>[4x]TEKKYIVALDQGTTSSRAVVMDHDANIISVSQREFEQIYPKPGWVEHDPMEIWATQSSTLVEVLTKADISSDQIAAIGITNQRETTIVWEKETGKPIYNAIVWQCRRTAEICEHLKRDGLEDYIRSNTGLVIDPYFSGTKVKWILDHV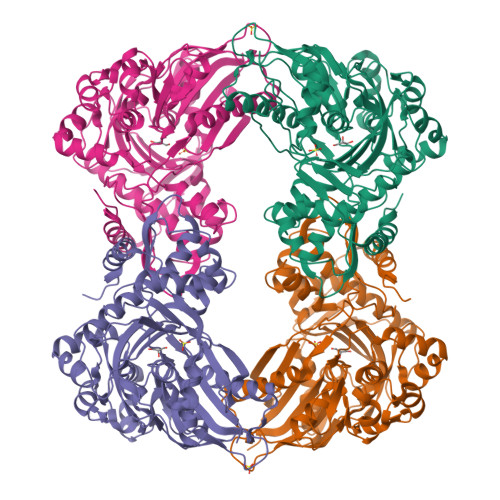EGSRERARRGELLFGTVDTWLIWKMTQGRVHVTDYTNASRTMLFNIHTLDWDDKMLEVLDIPREMLPEVRRSSEVYGQTNIGGKGGTRIPISGIAGDQQAALFGQLCVKEGMAKNTYGTGCFMLMNTGEKAVKSENGLLTTIACGPTGEVNYALEGAVFMAGASIQWLRDEMKLINDAYDSEYFATKVQNTNGVYVVPAFTGLGAPYWDPYARGAIFGLTRGVNANHIIRATLESIAYQTRDVLEAMQADSGIRLHALRVDGGAVANNFLMQFQSDILGTRVERPEVREVTALGAAYLAGLAVGFWQNLDELQEKAVIEREFRPGIETTERNYRYAGWKKAVKRAMAWEEHDE>[6x]STFVAKDGTQIYFKDWGSGKPVLFSHGWLLDADMWEYQMEYLSSRGYRTIAFDRRGFGRSDQPWTGNDYDTFADDIAQLIEHLDLKEVTLVGFSMGGGDVARYIARHGSARVAGLVLLGAVTPLFGQKPDYPQGVPLDVFARFKTELLKDRAQFISDFNAPFYGINKGQVVSQGVQTQTLQIALLASLKATVDCVTAFAETDFRPDMAKIDVPTLVIHGDGDQ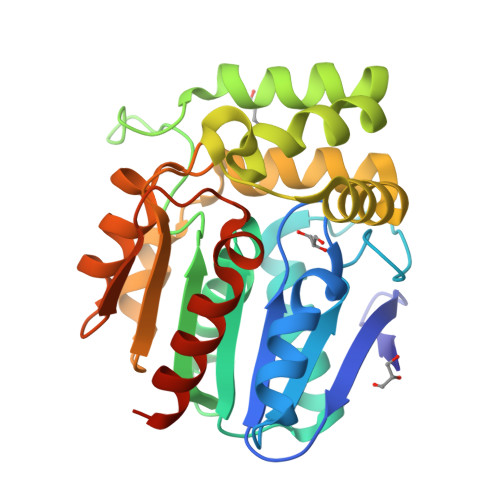IVPFETTGKVAAELIKGAELKVYKDAPHGFAVTHAQQLNEDLLAFLKRGSHHHHHH> MSRDRFRSRGGGGGGFHRRGGGGGRGGLHDFRSPPPGMGLNQNRGPMGPGPGGPKPPIPPPPPHQQQPQQPPPQQPPPQQPPPHQQPPPHQPPHQQPPPPPQDSSKPVVPQGPGSAPGVSPAPPPAGSAPPANPPTTGAPPGPGPTPTPPPAVTSATPGPPPPSTPSSGVSTTPPQSGGPPPPPAGGAGPGPKQGPGPGPGGPKGGKMPGGPKPGGGPGMGA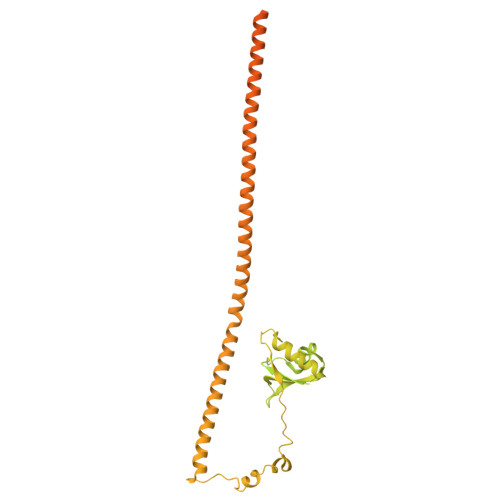PGGHPKPPHRGGGEPRGGRQHHPPYHQQHHQGPPPGGPAARTEEKISDSEGFKANLSLLRRPGEKTYTQRCRLFVGNLPADITEDEFKRLFAKYGEPGEVFINKGKGFGFIKLESRALAEIAKAELDDTPMRGRQLRVRFATHAAALSVRNLSPYVSNELLEEAFSQFGPIERAVVIVDDRGRSTGKGIVEFASKPAARKAFERCSEGVFLLTTTPRPVIVEPLEQLDDEDGLPEKLAQKNPMYQKERETPPRFAQHGTFEYEYSQRWKSLDEMEKQQREQVEKNMKDAKDKLESEMEDAYHEHQANLLRQDLMRRQEELRRMEELHSQEMQKRKEMQLRQEEERRRREEEMMIRQREMEEQMRRQREESYSRMGYMDPRERDMRMGGGGTMNMGDPYGSGGQKFPPLGGGGGIGYEANPGVPPATMSGSMMGSDMRTERFGQGGAGPVGGQGPRGMGPGTPAGYGRGREEYEGPNKKPRF> MTGVSDIQEAVAQIKAAGPSKPRLARDPVNQPMINNWVEAIGDRNPIYVDDAAARAAGHPGIVAP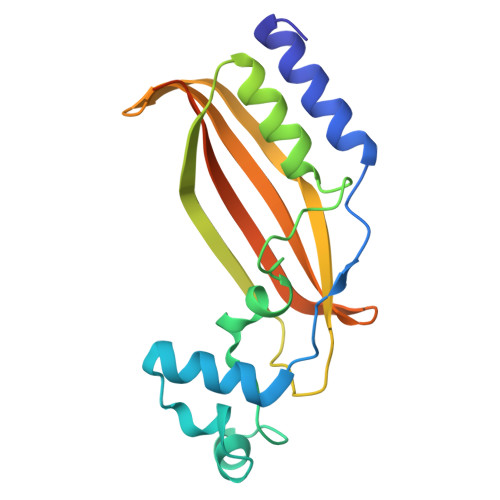PAMIQVWTMMGLGGVRPKDDPLGPIIKLFDDAGYIGVVATNCEQTYHRYLLPGEQVSISAELGDVVGPKQTALGEGWFINQHIVWQVGDEDVAEMNWRILKFKPAGSPSSVPDDLDPDAMMR> GGSMGKTADNHGPVRSETAREGRENQVYSPVTGARLVAGCICLTPDKKQVLMITSSAHKKRWIVPKGGVEKDEPNYETTAQRQTWEEAGCIGKIVANLGTVEDMRPPKDWNKDIKQFENSRKDSEVAKHPPRTEFHFYELEIENLLDKFPECHKRHRKLYSYTEAKQNLIDAKRPELLEALNRSAIIKDDK

The yeast diadenosine and diphosphoinositol polyphosphate phosphohydrolase DDP1 is a Nudix enzyme with pyrophosphatase activity on diphosphoinositides, dinucleotides, and polyphosphates. ScDDP1, like its human orthologs, adopts the canonical Nudix fold showing two β sheets flanked by helices. The active site lies in the crevice situated between both β sheets. The longest helix (α-1) contains the Nudix box (GX5EX7REUXEEXGU), which displays a β-loop-helix-loop structure that binds the Mg2+ ions involved in diphosphate moiety orientation and catalysis.

We have performed site-directed mutagenesis on Glu80, Glu83, and Arg32. Both mutants on acidic residues produce inactive forms of the enzyme or those with very low activity. While Glu80 binds Mg3 (its equivalent in HsDIPP1 also binds Mg2), Glu83 forms a triad structure with Arg79 and Glu80, fixing a perfect orientation of these residues. We crystallized inactive DDP1-E80Q in complex with 1-InsP7, showing also bm2 mode for the inositide; however, there is no Mg3 in the active site as expected, and, in consequence, the diphosphate moiety only fits in a nonproductive conformation. The DDP1-E80Q mutant precludes Mg3 binding, and, in consequence, it selects only the conformation of 1-InsP7 with its diphosphate bound solely to Mg1 (bottom). Mg3 is only present in wt-ScDDP1. E80Q and E83A impede the metal coordination and, in consequence the catalysis, but they have no effect in substrate binding as seen in this section.In this study, we focus on the ω-transaminase from Mycobacterium vanbaalenii (MvTA) which exhibits activity toward d-fructose rather than fructose 6-phosphate. The transaminase MvTA demonstrates transaminate activity toward d-fructose 1, and the resulting 2-amino-2-deoxy-mannitol (ADM) 2 undergoes dehydrogenation under the enzyme GutB1 and spontaneously cyclizes to produce the valuable azasugar mannojirimycin (MJ), which serves as a precursor for 1-DNJ. The dimeric enzyme exhibited the characteristic structural architecture of class IV PLP-dependent enzymes, consisting of two subunits. The interface between the two subunits constituted the binding pocket for the amino donor and acceptor.

A mutant M9 with significantly enhanced activity and thermostability has been successfully obtained and crystallized for structural resolution. Based on the level of thermostability improvement, the additional five mutation sites (S105P, S121M, H152N, A168E and R215G) were sequentially incorporated into M4, resulting in the generation of mutant M9. The activity of M9 was measured as 39.4 ± 1.5 mU/mg, demonstrating a remarkable 16.4-fold increase compared to that of WT. The half-life (t1/2) of M9 at 50°C represented a 208-fold improvement compared to WT. In all three structures, the asymmetric unit comprised two polypeptide chains forming a homodimer. For insatance, the Lys195, located on Loop2 (Chain A) and Loop4 (Chain B), served as the catalytic residue, and the flexible loops of Loop1 and Loop3 were likely involved in substrate binding. The results suggested that the mutations in residues surrounding the substrate binding pocket (L162I, H69K, K145R and K142P) had minimal impact on thermostability, while the mutations in residues positioned on the surface (S105P, S121M, H152N, A168E, and R215G) notably enhanced thermostability. Through further rational design using the crystal structure of M9, the mutant M9-1 with an additional 1.9-fold improvement in specific activity was obtained.

>[4x]MGIDTGTSNLVAVEPGAIREDTPAGSVIQYSDYEIDYSSPFAGGVAWIEGEYLPAEDAKISIFDTGFGKSDLTYTVAHVWHGNIFRLGDHLDRLLDGARKLRLDPGYTKDELADITKKCVMLSQLRESFVNLTITRGYGKRPGERDLSKLTNQVYIYAIPYIWAFPPEEQIFGTTAVVPRHVRRAGRNTVDPTIKNYQWGDLTAASFEAKDRGAGTAILMDADNCVAEGPGFNVCIVKDGKLASPSRNALPGITRKTVFEIAGAMGIEAALRDVTSHELYDADEIMAVTTAGGVTPINTLDGVPIGDGEPGPVTVAIRDRFWALMDEPGPLIEAIQY The U1A/U2B″/SNF family of RBPs is found in the U1 and/or U2 small nuclear ribonucleoprotein (snRNP) components of the spliceosome. Jawed vertebrates use U1A to bind stem-loop II of U1 snRNA (U1SLII) and U2B″ in conjunction with the leucine-rich repeat (LRR) protein U2A′ to bind SLIV of U2 snRNA (U2SLIV). Both U1A and U2B″ employ an N-terminal RNA recognition motif (RRM) to specifically recognize their RNA targets. Here, we report crystal structures of four states of dSNFRRM1 at 2 Å resolution or better: the free dSNFRRM1 (residues 1–96; dSNF1–96), dSNF1–96–dU1SLII, dU2A′–dSNF1–96, and dU2A′–dSNF1–96–dU2SLIV. Altogether with the characterization of dSNFRRM1 dynamics alone and in complexes by NMR spectroscopy and targeted mutagenesis combined with binding studies, we delineated how the intrinsic dSNFRRM1 RNA-binding capacity and specificity are fine-tuned by networks of intra-molecular interactions that modulate dSNFRRM1 dynamics, and how the auxiliary dU2A′ protein can capitalize on intrinsic dSNFRRM1 flexibility to gear dSNFRRM1 binding specifically to dU2SLIV.

We used a 22-residue, blunt-ended dU1SLII construct to determine the crystal structure of a dSNF1–96-dU1SLII complex at 2.0 Å resolution. dU1SLII contains a 10-nucleotide (nt) loop (A7-C16) closed by a C6:G17 Watson-Crick base pair (to simplify comparisons between the various RNAs, we numbered them identically according to the provided scheme). The center of the loop arches across the dSNF1–96 β-sheet, L3 protrudes through the RNA loop, while L1, L6, and α3 border the outside of the loop. In contrast in the Drosophila complex, the corresponding dSNFRRM1 residues (Leu43, Thr45, Lys44, and Lys47, respectively) do not allow the formation of a similarly extensive water network. While Thr45, Lys44, and Lys47 engage in water-mediated contacts to the phosphate oxygens of C16 and G17, a more expanded network is prevented by Leu43, which replaces Ser46 of hU1ARRM1 in dSNFRRM1. As a consequence, C14 can adopt two alternative conformations. In one conformation, it is bulged out and does not contact dSNFRRM1 (two of the three crystallographically independent complexes in the crystal); in the other, its base is flipped towards dSNFRRM1, where it rests on a hydrophobic surface formed by Val41 (β2) and Leu43 (L3) and where it engages in hydrogen bonds to the side chain of Lys24 (α1) and the backbone carbonyl group of Ile40 (β2; one of the crystallographically independent complexes). Lys47 (L3) contacts the phosphate on the 5′ side of A12 in the Drosophila complex, while the equivalent hU1ARRM1 Lys50 does not. While Asn12 (Asn15 in hU1ARRM1) hydrogen bonds to N7 of G10 in both organisms, it is stabilized by Gln80 (Arg83 in hU1ARRM1) only in Drosophila. Conversely, Ser84 in dSNFRRM1 engages in a hydrogen bond to the 6-amino group of A12, while the equivalent Ala88 of hU1ARRM1 cannot.

>[3x]GAMEMLPNQTIYINNLNEKIKKEELKKSLYAIFSQFGQILDIVALKTLKMRGQAFVIFKEIGSASNALRTMQGFPFYDKPMQIAYSKSDSDIVAKIKG> MEPAMEPETLEARINRATNP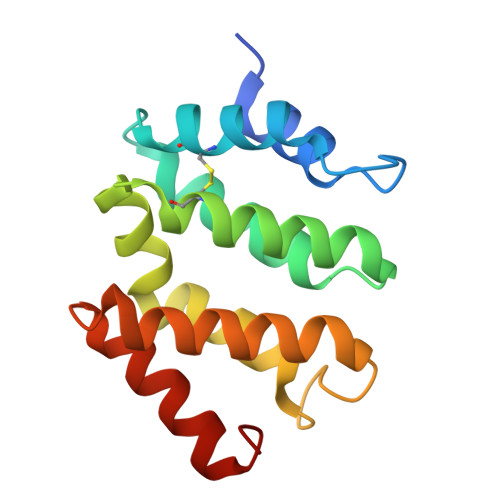LNKELDWASINGFCEQLNEDFEGPPLATRLLAHKIQSPQEWEAIQALTVLETCMKSCGKRFHDEVGKFRFLNELIKVVSPKYLGSRTSEKVKNKILELLYSWTVGLPEEVKIAEAYQMLKKQGIVKS> MIRNKAFVVRLYPNAAQTELINRTLGSARFVYNHFLARRIAAYKESGKGLTYGQTSSELTLLKQAEETSWLSEVDKFALQNSLKNLETAYKNFFRTVKQSGKKVGFPRFRKKRTGESYRTQFTNNNIQIGEGRLKLPKLGWVKTKGQQDIQGKILNVTVRRIHEGHYEASVLCEVEIPYLPAAPKFAAGVDVGIKDFAIVTDGVRFKHEQNPKYYRSTLKRLRKAQQTLSRRKKGSARYGKAKTKLARIHKRIVNKRQDFLHKLTTSLVREYEIIGTEHLKPDNMRKNRRLALSISDAGWGEFIRQLEYKAAWYGRLVSKVSPYFPSSQLCHDCGFKNPEVKNLA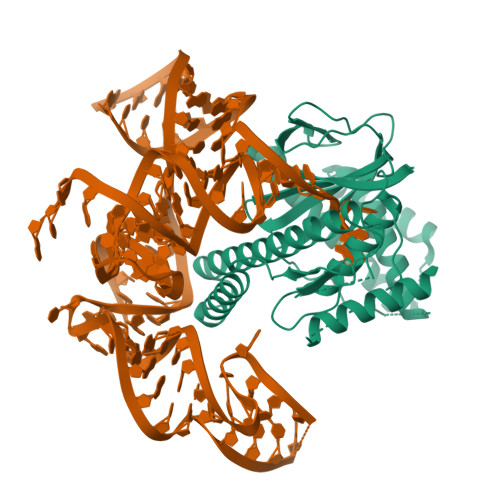VRTWTCPNCGETHDRDENAALNIRREALVAAGISDTLNAHGGYVRPASAGNGLRSENHATLVV5-(1,4-oxazepan-4-yl)pyridine-2-carbonitrile 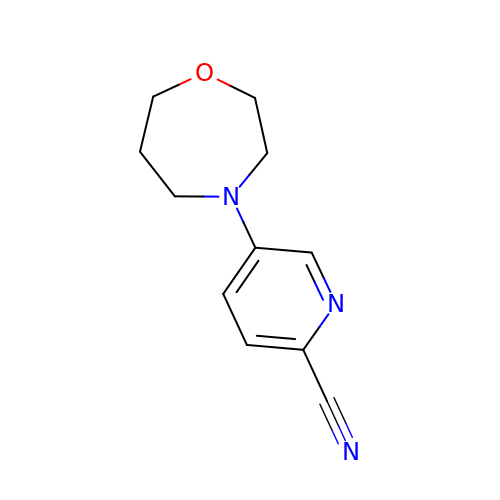| C11 H13 N3 O | QPJKHSFVBDONPD-UHFFFAOYSA-N> RRGSFVEMVDNLRGKSGQGYYVEMTVGSPPQTLNILVDTGSSNFAVGAAPHPFLHRYYQRQLSSTYRDLRKGVYVPYTQGKWEGELGTDLVSIPHGPNVTVRANI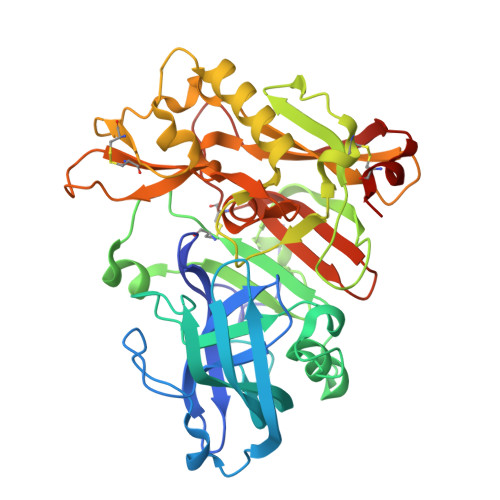AAITESDKFFINGSNWEGILGLAYAEIARPDDSLEPFFDSLVKQTHVPNLFSLQLCGAGFPLNQSEVLASVGGSMIIGGIDHSLYTGSLWYTPIRREWYYEVIIVRVEINGQDLKMDCKEYNYDKSIVDSGTTNLRLPKKVFEAAVKSIKAASSTEKFPDGFWLGEQLVCWQAGTTPWNIFPVISLYLMGEVTNQSFRITILPQQYLRPVEDVATSQDDCYKFAISQSSTGTVMGAVIMEGFYVVFDRARKRIGFAVSACHVHDEFRTAAVEGPFVTLDMEDCGYN> AEEELETPTPTQRGEAESRGDGLVDVMWEYKWENTGDAELYGPFTSAQMQTWVSEGYFPDGVYCRKLDPPGGQFYNS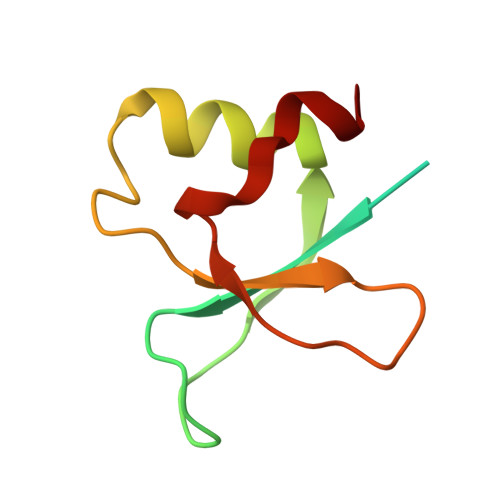KRIDFDLYT3-(1,3-BENZOTHIAZOL-2-YL)-2-(1,4-DIOXO-1,2,3,4-TETRAHYDROPHTHALAZIN-6-YL)-5-[(E)-2-PHENYLVINYL]-3H-TETRAAZOL-2-IUM | C24 H16 N7 O2 S | 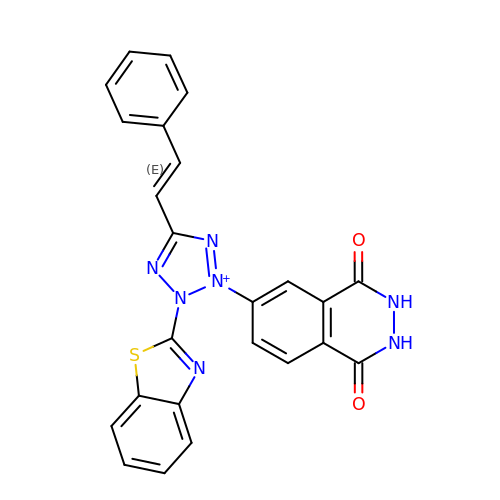BEIGFKLRGRRJJA-JLHYYAGUSA-O5-{5-chloro-4-[(5-cyclopropyl-1H-pyrazol-3-yl)amino]pyrimidin-2-yl}thiophene-2-sulfonamide 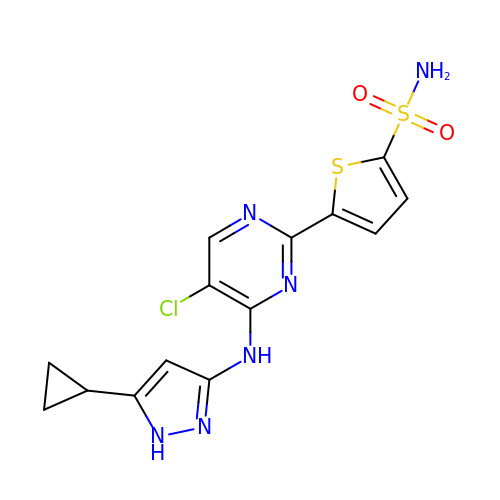| C14 H13 Cl N6 O2 S2 | KRMDPWLIHGQVGZ-UHFFFAOYSA-N> PRRAREYPEEGEFVVATVKRIHNYGAFLELDEYPGKEAFMHISEVASTWVRNIRDYLKEGQKVVAKVIR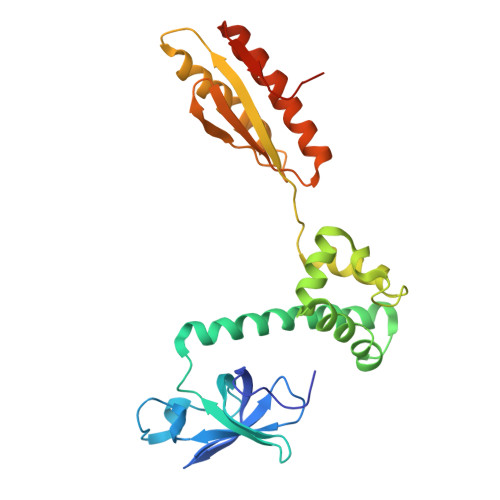VDPRKGHIDLSLRRVTQQQRKAKLQEFKRAQKAENLLKLAAEKLGKDFETAWREVWVPLEEEWGEVYAAFEDAAKDGIDVLKGHVPDEWLPVLKEIIDNYVEVPTVTIDAEFEITVPKPNGVEIIKEALIRARDRANKEKDVEVKFTYLGAPRYRIDITAPDYYKAEEVLESIAEEILRVIKEAGGEATLLRKEKRIKKVKKRKK>[2x]HLKQIEKVKKLDKWVPHELTENQKNRRFEVSSSLILRNHNEPFLDRIVTCDEKWILYDNRRRSAQWLDQEEAPKHFPKP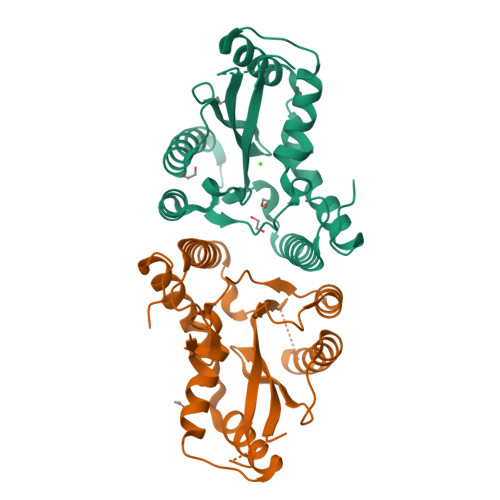ILHPKKVMVTIWWSAAGLIHYSFLNPGETITSEKYAQEIDEMNQKLQRLQLALVRRKRPILLHDNARPHVAQPTLQKLNELGYEVLPHPPYSPDLLPTNYHVFKHLNNFLQGKRFHNQQDAENAFQEFVESQSTDFYWTGINQLISRWQKCVDCNGSYFD>[12x]MGSSHHHHHHSQDPNSMKSEPLSYLGKDGGPWEIFTEQVDRVVPYLGRLAPLAESLKRPKRVLIVDVPVRLDDGSVAYFEGYRVHHNTARGPAKGGVRYHPEVTLSEVMALAGWMTIKNAA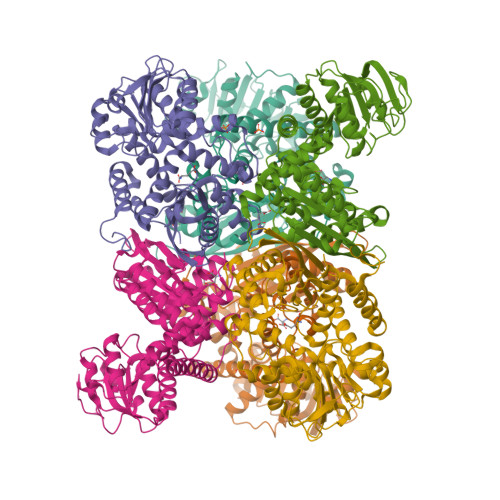VGLPYGGGKGGIRVDPRKLSPGELERLTRRYTSEIGILLGPDRDIPAPDVNTGEREMAWMMDTYSMNVGRTVPGVVTGKPIALGGSLGRRDATGRGVFITAAAAAEKIGLQVEGARVAIQGFGNVGNAAARAFHDHGARVVAVQDHTGTVYNEAGIDPYDLLRHVQEFGGVRGYPKAEPLPAADFWGLPVEFLVPAALEKQITEQNAWRIRARIVAEGANGPTTPAADDILLEKGVLVVPDVIANAGGVTVSYFEWVQDFNSYFWTEEEINARLERVLRNAFEAVWQVAQEKKIPLRTAAYVVAATRVLEARALRGLYP>[2x]MTVQMEYEKDVKVAALDGKKIAVIGYGSQGHAHAQNLRDSGRDVIIGVEPGKSFDKAKEDGFDTYTVAEATKLADVIMILAPDEIQQELYEAEIAPNLEAGNAVGFAHGFNIHFEFIKVPADVDVFMCAPKGPGHLVRRT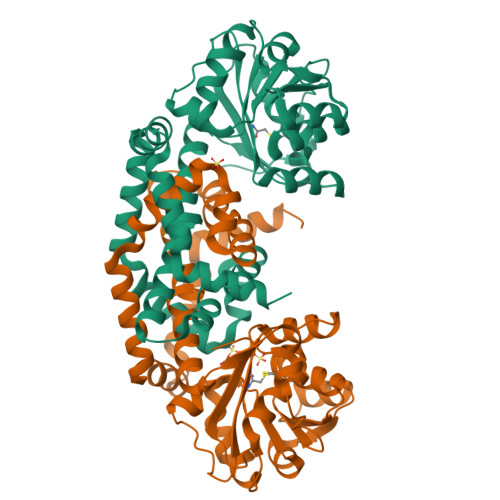YEEGFGVPALYAVYQDATGNAKNIAMDWCKGVGAARVGLLETTYKEETEEDLFGEQAVLCGGLTALIEAGFEVLTEAGYAPELAYFEVLHEMKLIVDLIYEGGFKKMRQSISNTAEYGDYVSGPRVITEQVKENMKAVLADIQNGKFANDFVNDYKAGRPKLTAYREQAANLEIEKVGAELRKAMPFVGKNDDDAFKIYN>MSLGKFLVEREQMRYPVDVYTGKIQAYPEGKPSAIAKIQVDGELMLTELGLEGDEQAEKKVHGGPDRALCHYPREHYLYWAREFPEQAELFVAPAFGENLSTDGLTESNVYMGDIFRWGEALIQVSQPRSPCYKLNYHFDISDIAQLMQN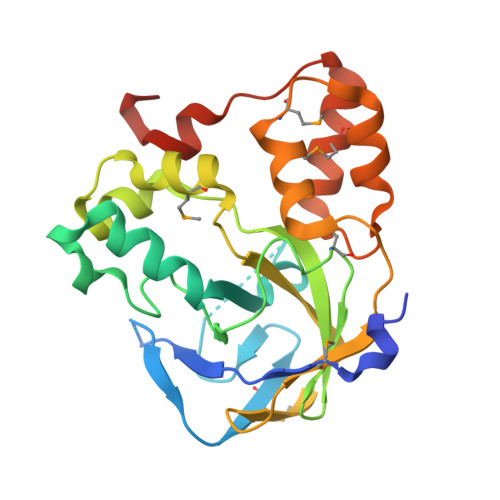TGKVGWLYSVIAPGKVSADAPLELVSRVSDVTVQEAAAIAWHMPFDDDQYHRLLSAAGLSKSWTRTMQKRRLSGKIEDFSRRLWGKEGGSHHHHHH[3x]>CGAATUCG[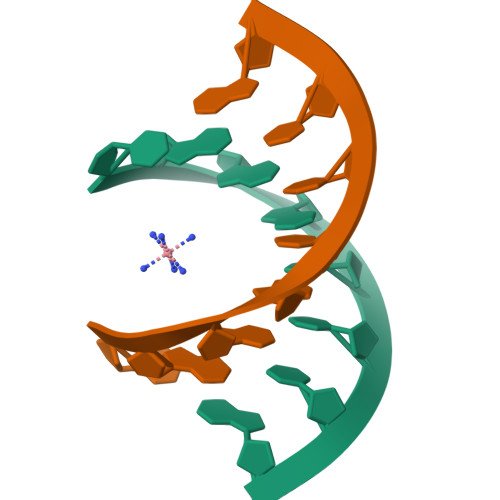4x]>[2x]MLILATLGSDKSVTTINAILTEIFTGLNPNKIIIFREDPQKKDIKGMEKALEYLGVNTLIEEKVIGEGIKLWREKIRNEEIDIFDITPGRKYMALSATYYSRAEEIRYVYLKDEREGYNIFGYVPFEQLKVINVRIGDEIPYDPPLTQNVNEAESLLDVDSLRAFINILGLHGKVEINGIDLENPDQVEEICLFRSGKYKYEEEKDIIKEAERGSLFLADTNVYIRLGNRLRSLVYN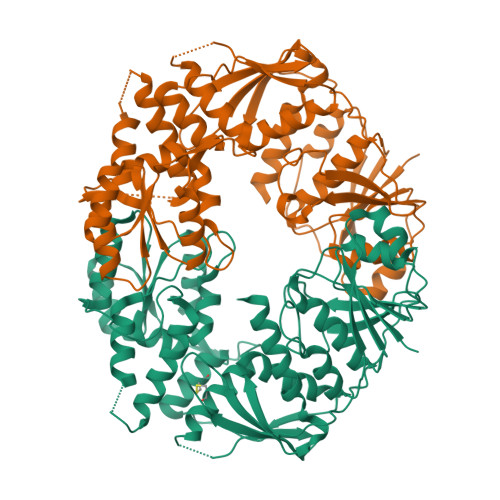RKYGFRLLSSKNTFNELYNHTAQDTQKIDENKVKFILGMLSYRSLHVPPITSQVRSSGDMGLINEALEIKKNVEDNVVLITADKALGLTAQSKGLRTIILSKVRKEIGEWDIGELLFCLSFYNDYRNGIRRMIEISLNGSKIAELHSYYHLQERRVKVRVVDKRYNYPKILEILSEILATADQAAAHHHHHH>IISRNFPIIGVKEKTFEQLHKKCLEKKVLYVDPEFPPDETSLFYSQKFPIQFVWKRPPEICENPRFIIDGANRTDICQGELGDAWFLAAIACLTLNQHLLFRVIPHDQSFIENYAGIFHFQFWRYGEWVDVVIDDCLPTYNNQLVFTKSNHRNEFWSALLEKAYAKLHGSYEALKGGNTTEAMEDFTGGVAEFFEIRDAPSDMYKIMKKAIERGSLMGCSIDDGTNMTYGTSPSGLNMGELIARMVRNMDNSLLQDSDLDPRGSDERPTRTIIPVQYETRMACGLVRGHAYSVTGLDEVPFKGEKVKLVRLRNPWGQVEWNGSWSDRWKDWSFVDKDEKARLQHQVTEDGEFWMSYEDFIYHFTKLEICNLTADLEHHH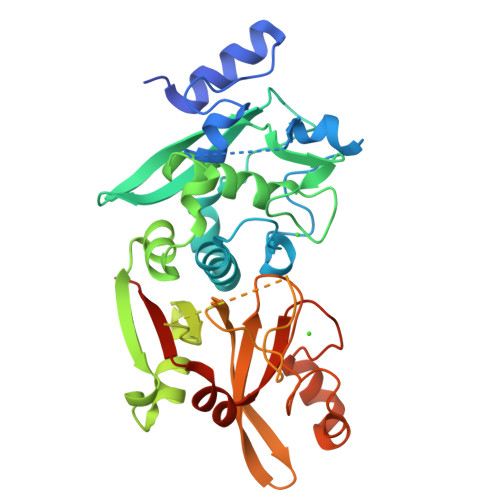HHH[4x]9-O-3'-quinolinium propylberberine 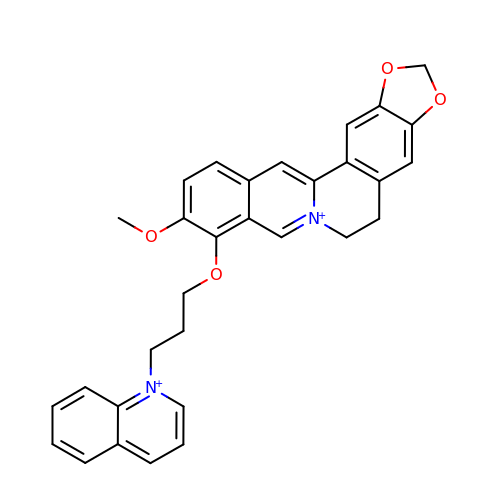| C31 H28 N2 O4 | NCXCLFQYKFLSTH-UHFFFAOYSA-N>GCAGC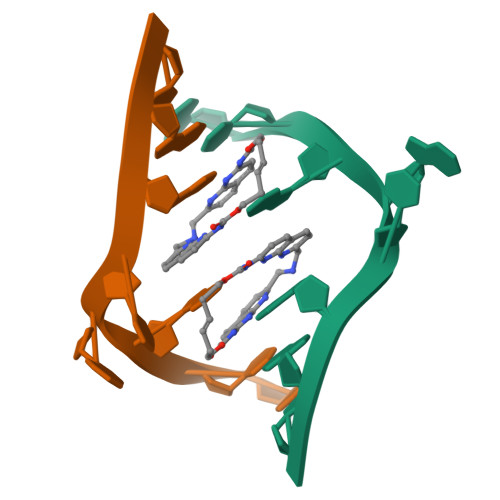AGC[8x]>MAQGNNYGQTSNGVADESPNMLVYRKMEDVIARMQDEKNGIPIRTVKSFLSKIPSVFSGSDIVQWLIKNLTIEDPVEALHLGTLMAAHGYFFPISDHVLTLKDDGTFYRFQTPYFWPSNCWEPENTDYAVYLCKRTMQNKARLELADYEAESLARLQRAFARKWEFIFMQAEAQAKVDKKRDKIERKILDSQERAFWDVHRPVPGCVNTTEVDIKKSSRMRNPHKTRKSVYGLQNDIRSHSPTHTPTPETKPPTEDELQQQIKYWQIQLDRHRLKMSKVADSLLSYTEQYVEYDPFLAPPDPSNPWLSDDTTFWELEASKEPSQQRVKRWGFGMDEALKDPVGREQFLKFLESEFSSENLRFWLAVEDLKKRPIREVPSRVQEIWQEFLAPGAPSAINLDSKSYDKTTQNVKEPGRYTFEDAQEHIYKLMKSDSYPRFIRSSAYQE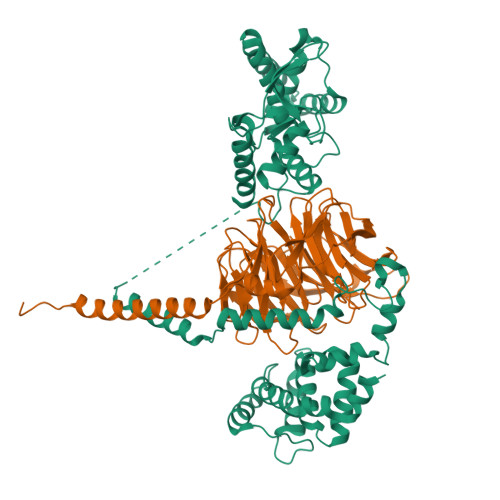LLQAKKKGKSLTSKRLTSLVQSY[2x];>MATDGLHENETLASLKSEAESLKGKLEEERAKLHDVELHQVAERVEALGQFVMKTRRTLKGHGNKVLCMDWCKDKRRIVSSSQDGKVIVWDSFTTNKEHAVTMPCTWVMACAYAPSGCAIACGGLDNKCSVYPLTFDKNENMAAKKKSVAMHTNYLSACSFTNSDMQILTASGDGTCALWDVESGQLLQSFHGHGADVLCLDLAPSETGNTFVSGGCDKKAMVWDMRSGQCVQAFETHESDVNSVRYYPSGDAFASGSDDATCRLYDLRADREVAIYSKESIIFGASSVDFSLSGRLLFAGYNDYTINVWDVLKGSRVSILFGHENRVSTLRVSPDGTAFCSGSWDHTLRVWA[2x]>GPDSSLFAPYLPQANIPELIQEGRLVAGILRVNKKNRSDAWVSTDGALDADIYICGSKDRNRALEGDLVAVELLVVDDVWESKKEKEEKKRRKDASMQHDLIPLNSSDDYHNDASVTAATSNNFLSSPSSSDSLSKDDLSVRRKRSSTINNDSDSLSSPTKSGVRRRSSLKQRPTQKKNDDVEVEGQSLLLVEEEEINDKYKPLYAGHVVAVLDRIPGQLFSGTLGLLRPSQQANSDNNKPPQSPKIAWFKPTDKKVPLIAIPTELAPKDFVENADKYSEKLFVASIKRWPITSLHPFGILVSELGDIHDPDTEIDSILRDNNFLSNEYLDQKNPQKEKPSFQPLPLTAESLEYRRNFTDTNEYNIFAISELGWVSEFALHVRNNGNGTLELGCHVVDVTSHIEEGSSVDRRARKRSSAVFMPQKLVNLLPQSFNDELSLAPGKESATLSVVYTLDSSTLRIKSTWVGESTISPSNILSLEQLDEKLSTGSPTSYLSTVQEIARSFYARRINDPEATLLPTLSLLESLDDEKVKVDLNILDRTLGFVVINEIKRKVNSTVAEKIYTKLGDLALLRRQMQPIATKMASFRKKIQNFGYNFDTNT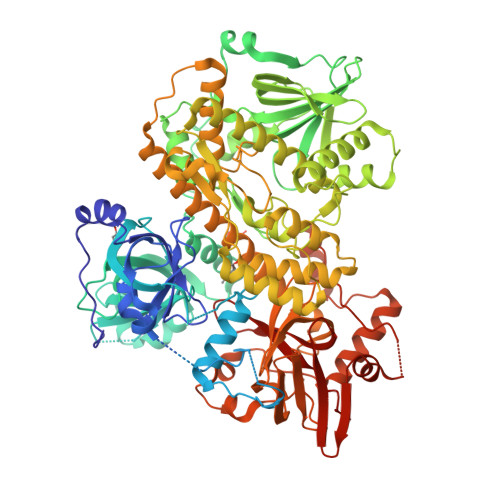ADELIKGVLKIKDDDVRVGIEILLFKTMPRARYFIAGKVDPDQYGHYALNLPIYTHFTAPMRRYADHVVHRQLKAVIHDTPYTEDMEALKITSEYCNFKKDCAYQAQEQAIHLLLCKTINDMGNTTGQLLTMATVLQVYESSFDVFIPEFGIEKRVHGDQLPLIKAEFDGTNRVLELHWQPGVDSATFIPADEKNPKSYRNSIKNKFRSTAAEIANIELDKEAESEPLISDPLSKELSDLHLTVPNLRLPSASDNKQNALEKFISTTETRIENDNYIQEIHELQKIPILLRAEVGMALPCLTVRALNPFMKRV[2x]> GLTEEQRMMIRELMDAQMKTFDTTFSHFKNFRLPGVLSSGCELPESLQAPSRE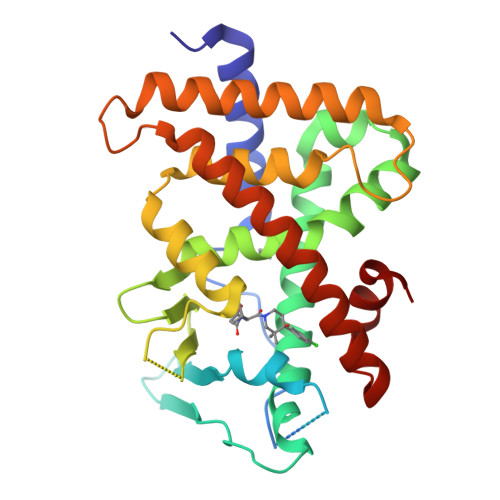EAAKWSQVRKDLCSLKVSLQLRGEDGSVWNYKPPADSGGKEIFSLLPHMADMSTYMFKGIISFAKVISYFRDLPIEDQISLLKGAAFELCQLRFNTVFNAETGTWECGRLSYCLEDTAGGFQQLLLEPMLKFHYMLKKLQLHEEEYVLMQAISLFSPDRPGVLQHRVVDQLQEQFAITLKSYIECNRPQPAHRFLFLKIMAMLTELRSINAQHTQRLLRIQDIHPFATPLMQELFGI>ANPNHPLLKKILMKAPGTYHHSMMVANLAEACADKIGANSLLVRVGCFYHDIGKTLRPPYFVENQLQGINPHDRLTPEQSRDIILSHTKDGAEILKENHMPQPIIDIALQHHGTTLLKYFYFKAKETNPDVKEADYRYSGP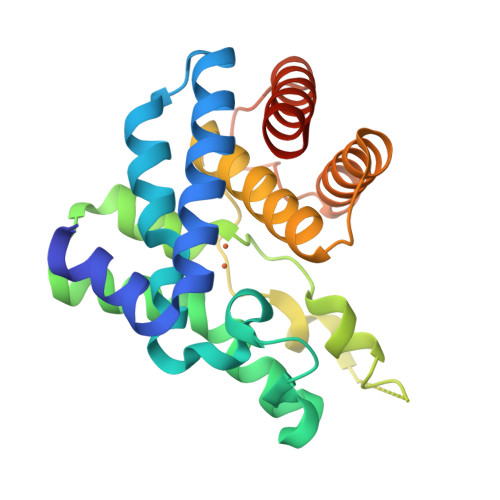KPQTKEIAIINISDSVEAAVRSSTEPTMAKITEIIDGIIKDRFLDGQFTECDITIQEIKIIRDTLIATLNGIYHQRIQYPD[2x]>ECQPIFLNVLEAIEPGVVCAGHDNNQPDSFAALLSSLNELGERQLVHVVKWAKALPGFRNLHVDDQMAVIQYSWMGLMVFAMGWRSFTNVNSRMLYFAPDLVFNEYRMHKSRMYSQCVRMRHLSQEFGWLQITPQEFLCMKALLLFSIIPVDGLKNQKFFDELRMNYIKELDRIIACKRKNPTSCSRRFYQLTKLLDSVQPIARELHQFTFDLLIKSHMVSVDFPEMMAEIISVQVPKILSGKVKPIYFHTQ[4x];>MSD[4x];>SLQFLLDT[4x]

The androgen receptor (AR/NR3C4) belongs to the steroid receptor subfamily of nuclear receptors (NRs), which also includes the glucocorticoid receptor (GR/NR3C1), mineralocorticoid receptor (MR/NR3C2), progesterone receptor (PR/NR3C3) and oestrogen receptors α and β (ERα/NR3A1; ERβ/NR3A2). The AR, in particular, is critically important for normal development and homeostasis of male and female reproductive organs and their physiology. Structurally, the AR is similar to other NRs consisting of an N-terminal domain, followed by an almost strictly conserved DNA-binding domain (DBD), an interdomain linker or hinge, and a C-terminal ligand-binding domain (LBD). The LBD contains the internal ligand-binding pocket (LBP) and two major solvent-exposed surfaces responsible for interaction with coregulators, activation function 2 (AF-2) and binding function 3 (BF-3)891011 and Supplementary References.

Here we present the crystal structure of the human AR-LBD homodimer bound to its natural agonist, dihydrotestosterone (DHT) and provide in addition strong evidence for its crucial role in receptor functioning. A synthetic UBA3 peptide comprising this motif, S59TESLQFLLDTCKV72 (S59-V72), was found by surface plasmon resonance (SPR) to bind with high affinity to liganded AR-LBD (KD=30.6±0.7 nM). Crystals of AR-LBD grown in the presence of this peptide diffracted X-rays up to a resolution of 2.15 Å, which allowed solution and refinement of the structure of the complex. Electron densities in and around coactivator binding AF-2 grooves could be safely interpreted as corresponding to residues S62-T69 of the UBA3 peptide. These residues adopt an α-helical conformation with the side chains of Leu residues L63 and L67 inserted into the AF-2 pockets of the AR-LBD, similar to the structures documented before for other LxxLL peptide motifs. All AR-LBD structures deposited in the Protein Data Bank (PDB) to date belong to the same crystal form (orthorhombic space group P212121), and feature a monomer in the asymmetric unit (ASU)20212223 and Supplementary References. In contrast, the current AR-LBD crystal structure belongs to the monoclinic space group (C2) and presents four independent, helically arranged LBD molecules in the ASU (details of the final electron density map are shown in Fig. 1c,d). Two of these LBD monomers form a symmetrical ‘core dimer' upon burial of ≈1,000 Å2 of solvent-exposed surface from each molecule, while two peripheral AR-LBDs associate more loosely to the BF-3 grooves of each of these monomers. Core dimer: the two monomers in the AR-LBD core dimer are arranged ‘head-to-head' around a local pseudo twofold axis with both AF-2 pockets facing opposite directions and separated by over 60 Å. The protein–protein interface is centred on residues from helix H5 and the L5-S1 loops of both partners, with additional contributions made by residues from H1 and H7-H9, L1–3, and β-strand S1.(2Z)-4-(dimethylamino)-N-{7-fluoro-4-[(2-methylphenyl)amino]imidazo[1,5-a]quinoxalin-8-yl}-N-methylbut-2-enamide | C24 H25 F N6 O | 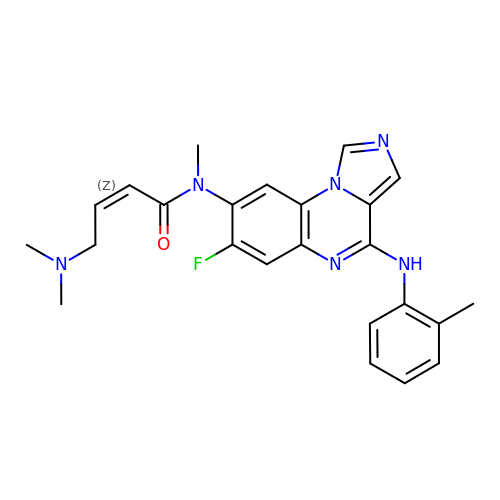YMSXHRWUGLAAKL-YFHOEESVSA-N> APSPLYSVEFSEEPFGVIVHRQLDGRVLLNTTVAPLFFADQFLQLSTSLPSQYITGLAEHLSPLMLSTSWTRITLWNRDLAPTPGANLYGSHPFYLALEDGGSAHGVFLLNSNAMDVVLQPSPALSWRSTGGILDVYIFLGPEPKSVVQQYLDVVGYPFMPPYWGLGFHLCRWGYSSTAITRQVVENMTRAHFPLDVQWNDLDYMDSRRDFTFNKDGFRDFPAMVQELHQGGRRYMMIVDPAISSSGPAGSYRPYDEGLRRGVFITNETGQPLIGKVWPGSTAFPDFTNPTALAWWEDMVAEFHDQVPFDGMWIDMNEPSNFIRGSEDGCPNNELENPPYVPGVVGGTLQAATICASSHQFLSTHYNLHNLYGLTEAIASHRALVKARGTRPFVISRSTFAGHGRYAGHWTGDVWSSWEQLASSVPEILQFNLLGVPLVGADVCGFLGNTSEELCVRWTQLGAFYPFMRNHNSLLSLPQEPYSFSEPAQQAMRKALTLRYALLPHLYTLFHQAHVAGETVARPLFLEFPKDSSTWTVDHQLLWGEALLITPVLQAGKAEVTGYFPLGTWYDLQTVPIEALGSLPPPPAAPREPAIHSEGQWVTLPAPLDTINVHLRAGYIIPLQGPGLTTTESRQQPMALAVALTKGGEARGELFWDDGESLEVLERGAYTQVIFLARNNTIVNELVRVTSEGAGLQLQKVTVLGVATAPQQVLSNGVPVSNFTYSPDTKVLDICVSLLMGEQFLVSWC;> QCDVPPNSRFDCAPDKAITQEQCEARGCCYIPAKQGLQGAQMGQPWCFFPPSYPSYKLENLSSSEMGYTATLTRTTPTFFPKDILTLRLDVMMETENRLHFTIKDPANRRYEVPLETPRVHSR

We developed and applied fluorescent activity-based probes reporting on either human GH30 lysosomal glucosylceramidase (GBA1, a retaining β-glucosidase) or GH31 lysosomal retaining α-glucosidase (GAA). Gaucher disease is rooted in genetic deficiency of the retaining β-glucosidase GBA1 (glucosylceramidase, glucocerebrosidase, member of the glycoside hydrolase (GH)30 superfamily of glycoside hydrolases)10 and Pompe disease is caused by genetic deficiency of the retaining α-glucosidase, GAA (member of the GH31 family). GBA1 and GAA produce glucose, but do so from different substrates and by following distinct reaction itineraries. However, and as dictated by the opposite (compared to glucosylceramide) anomeric configuration, it does so following the reverse reaction itinerary: 4C1 → [4H3]‡ → 1S3. Both GBA1 and GAA-mediated hydrolyses proceed through a flattened 4H3 transition state, a feature that, in combination with the occurrence of a covalent intermediate, can be capitalised on for the design of covalent inhibitors and activity-based probes (ABPs).

GAA processes its substrate, glycogen (α-1,4/1,6-linked glucopyranose polymers), in a related Koshland double displacement mechanism. 1,6-Epi-cyclophellitol in turn is a mechanism-based retaining α-glucosidase inhibitor. Substitution of the primary alcohol in 1,6-epi-cyclophellitol for a reporter is not an option – inhibitory potency will be lost – and the same holds true for any of the three secondary alcohols. Substitution of the epoxide oxygen for an aziridine nitrogen and installation of a reporter on this nitrogen, as depicted in Fig. 1d, does yield an effective activity-based probe that, while not GAA selective, is in general in-class selective for retaining α-glucosidases. Ensuing copper(i)-catalysed azide–alkyne [2 + 3] cycloaddition with TAMRA-alkyne yielded GAA ABP II. More broadly speaking, the work described here also reveals that substitution of the Bodipy-type dyes we routinely install on our cyclophellitol ABPs as reporter entities, for the TAMRA dye (commonly used in FluoPol-based assays) is not detrimental for probe affinity. We confirmed this also by crystal structures, with as examples (in the ESI†) the covalent complex of rhGBA1 reacted with a previously reported Bodipy variant of ABP I as well as that of rhGAA reacted with TAMRA-ABP II.> AKPAAENLSLVVHGPGDLRLENYPIPEPGPNEVLLKMHSVGICGSDVHYWQHGRIGDFVVKKPMVLGHEA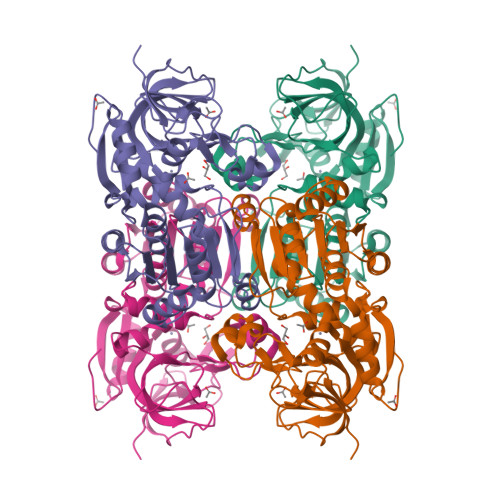SGTVVKVGSLVRHLQPGDRVAIQPGAPRQTDEFCKIGRYNLSPTIFFCATPPDDGNLCRFYKHNANFCYKLPDNVTFEEGALIEPLSVGIHACRRAGVTLGNKVLVCGAGPIGLVNLLAAKAMGAAQVVVTDLSASRLSKAKEVGADFILEISNESPEEIAKKVEGLLGSKPEVTIECTGVETSIQAGIYATHSGGTLVLVGLGSEMTSVPLVHAATREVDIKGVFRYCNTWPMAISMLASKSVNVKPLVTHRFPLEKALEAFETSKKGLGLKVMIKCDPSDQNP> GPAMLPISMSDEGDSFLVKDSLGENKIPKNPSKVVIL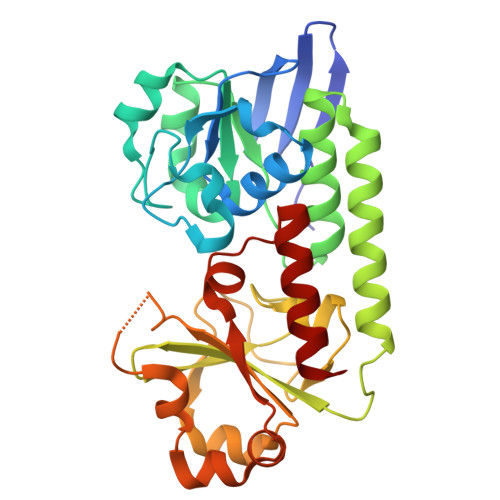DLGILDTFDALKLNDKVVGVPAKNLPKYLQQFKNKPSVGGVQQVDFEAINALKPDLIIISGRQSKFYDKLKEIAPTLFVGLDNANFLSSFENNVLSVAKLYGLEKEALEKISDIKNEIEKAKSIVDEDKKALIILTNSNKISAFGPQSRFGIIHDVLGINAVDENIKVGTAGKSINSEFILEKNPDYIFVVDRNVILGNKERAQGILDNALVAKTKAAQNKKIIYLDPEYWFLASGNGLESLKTMILEIKNAVK> GQVAPNVWSKYFNIPNPGLRAYFSNVVSGQPEVYRTPFYKGMSLESICDEWYKKLVSIDTQWPTLMEFEDDLRKKVGPMSVMLPLKERMSDIDSYYDSISKDQVPFDTKAISAAKSEWKGVSRLRLRSEVNTVAVMKKSTNSGSPYFSKRKAVVSKTIPCDVYMDGRYCVMRQNGREWSGAAVLGWRGQEGGPKPTDVKQRVVWMFPFAVNIRELQVYQPLILTFQRLGLVPAWVSMEAVDRRITKMFDTKGPRDVVVCTDFSKFDQHFNPTCQSVAKELLADLLTGQEAVDWLERVFPIKYAIPLAYNWGEIRYGIHGMGSGSGGTNADETLVHRVLQHEAAISHHTTLNPNSQCLGDDGVLTYPGISAEDVMQSYSRHGLDMNLEKQYVSKQDCTYLRRWHHTDYRVDGMCVGVYSTMRALGRLAMQERYYDPDVWGEKMVTLRYLSIIENVKYHPLKEEFLDFCIKGDKTRLGLGIPGFLDNIAGEAQKAIDMMPDFLGYTKSLQYDGDLRRNAAAGIENWWVVQALKSRR

Picobirnaviruses (PBV) are small, non-enveloped dsRNA viruses infecting a wide range of mammalian and avian species. Human PBV (hPBV) has been identified on almost every continent, and has been associated with acute gastroenteritis primarily in children and people that are immunocompromised. It has a bi-segmented genome with the genome segment two (PBV2) encoding the viral RdRP and the genome segment one (PBV1) encoding the CP and a protein of unknown function. The hPBV RdRP possesses a canonical polymerase fold with a 24 amino acids (aa) long C-terminal insertion loop structure that partially occupies the active site of the polymerase. The polymerase domain, which is structurally highly conserved amongst RNA viruses, has a right-hand configuration with three subdomains: the fingers (aa 85–230, 268–324), palm (aa 231–267, 325–414), and thumb (aa 415–470).

To determine the exact biological function of the insertion loop structure, a hPBV RdRP lacking the loop structure (i.e. ΔLOOP) was synthesized and expressed. Gel filtration chromatography showed that ΔLOOP was eluted at a similar position as the WT protein. The ΔLOOP RdRP was crystallized and its structure solved by molecular replacement using the WT RdRP structure as the phasing model. The overall structure of ΔLOOP appears to be essentially the same as the WT RdRP (root-mean-square deviation in distance = 0.4 Å for 3275 common atoms), except for the deleted insertion loop which became unstructured in the ΔLOOP RdRP. Given this structural information, we are confident that the removal of the insertion loop should not affect the overall folding of the polymerase, and that the ΔLOOP RdRP should provide an excellent tool to study the function of the insertion loop structure using in vitro assays. However, while the WT RdRP utilizes a de novo initiation mechanism for RNA synthesis, the ΔLOOP could only initiate RNA replication through back-priming, suggesting that the insertion loop serves as a platform for initiation. Due to the heat denaturation, the dsRNA products generated by the WT RdRP were converted to ssRNA, while the dsRNA products of the ΔLOOP RdRP retained the same mobility as the original dsRNA. This result indicates that back-priming was taking place during dsRNA synthesis by the ΔLOOP RdRP, thus producing a product that was covalently linked to the ssRNA template. Additionally, it was noted that the removal of the insertion loop significantly increased the TNTase activity of the RdRP. Given our TNTase activity data and the fact that the insertion loop is located near the C-terminus of the hPBV RdRP, we propose that the removal of the insertion loop structure leaves the dsRNA exit channel of the protein permanently open, thus allowing the 3’-end of the RNA molecules to reach the active site for nucleotidyl addition in an orientation that is compatible for nucleotide addition.> FQQLSARLQEAIGRLRGRGRITEEDLKATLREIRRALMDADVNLEVTRDFVERVREEALGKQVLESLTPAEVILATVYEALKEALGGEARLPVLKDRNLWFLVGLQGSGKTTTAAKLALYYKGKGRRPLLVAADTQRPAAREQLRLLGEKVGVPVLEVMDGESPESIRRRVEEKARLEARDLILVDTAGRLQIDEPLMGELARLKEVLGPDEVLLVLDAM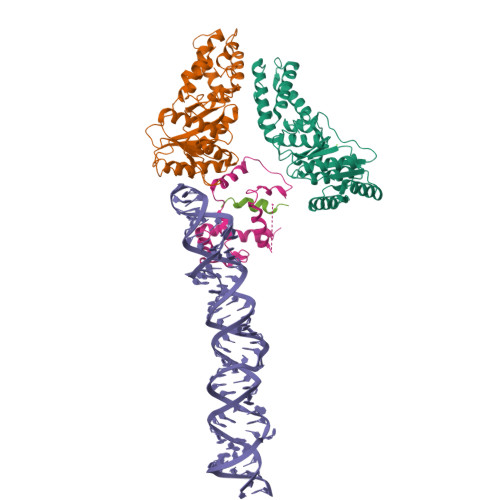TGQEALSVARAFDEKVGVTGLVLTKLDGDARGGAALSARHVTGKPIYFAGVSEKPEGLEPFYPERLAGRILGMG;> RSLLKTKENLGSGFISLFRGKKIDDDLFEELEEQLLIADVGVETTRKIITNLTEGASRKQLRDAEALYGLLKEEMGEILAKVDEPLNVEGKAPFVILMVGVNGVGKTTTIGKLARQFEQQGKSVMLAAGDTFRAAAVEQLQVWGQRNNIPVIAQHTGADSASVIFDAIQAAKARNIDVLIADTAGRLQNKSHLMEELKKIVRVMKKLDVEAPHEVMLTIDASTGQNAVSQAKLFHEAVGLTGITLTKLDGTAKGGVIFSVADQFGIPIRYIGVGERIEDLRPFKADDFIEALFAR;> LEEYDKIQKKMEDVMEGKGKLTLRDVYAQIIALRKMGPLSKVLQHIPGLGIMLPTPSEDQLKIGEEKIRRWLAALNSMTYKELENPNIIDKSRMRRIAEGSGLEVEEVRELLEWYNNMNRLLKMV;> GIILVLLIWGTVLL Interleukin 4 (IL-4) is a pleiotropic cytokine that plays a major regulatory role in the immune system. Signal transduction of IL-4 is mediated by a sequential binding process, initiated first by binding of IL-4 to its high-affinity single membrane spanning receptor chain IL-4Rα. This intermediate ligand receptor complex then recruits one of two possible low-affinity receptor subunits, the common gamma chain (γc) or the IL-13Rα1 chain, into the functional hetero-trimeric complex to initiate signalling. The overall structure of IL-4 comprises the known four-helical bundle in up-up-down-down topology, which like the crystal packing is unaffected by these mutations.

Analysis of the variants T13D and F82D yielded dissociation constants KD of 0.02 – 0.04 nM and 0.03 – 0.04 nM respectively. The structures of the IL-4 variants T13D (max. resolution 1.65 Å), F82D (max. resolution 1.7Å) and T13D-F82D (max. resolution 1.8Å) were refined on the basis of the structure of wild-type IL-4 (max. resolution 1.8Å); all crystals were obtained under identical conditions, allowing detailed comparison. The structure of the super-agonist variant F82D shows a different picture; the side chain conformation, i.e. the χ1 and χ2 torsion angles, of Asp82 is identical to that of the wild-type Phe82. Interestingly, the high-resolution structure of variant F82D reveals two alternative side chain conformations for Arg85. In one, the side chain is not hydrogen-bonded to the Asp residue introduced at position 82 and is oriented towards the solvent. In the second, the side chain interacts with the carboxylate group of Asp82 via a weak single hydrogen bond, but it is much less fixed than in the variant T13D. The distance between the amino group of Arg85 and the carboxylate group of Asp82 is 3.2Å and therefore close to the exclusion criterion for a hydrogen bond. In addition, the temperature factors of the Arg85 side chain atoms are elevated compared to those of rigid main chain or side chain atoms in the variant F82D, indicating that the stabilization of a certain side chain conformation is not as rigid as in variant T13D. The model of the F82D:IL-4Rα complex allows us to propose a stabilizing mechanism similar to that suggested for the complex of T13D and IL-4Rα. Here, too, the carboxylate group of Asp82 (F82D) forms a bi-dentate salt bridge with the guanidinium group of Arg85, thereby immobilizing the side chain of Arg85 in the ligand-receptor interface.

> HKCDITLQEIIKTLNSLTEQKTLCTELTVTDIFAASKNTTEKETFCRAATVLRQFYSHHEKDTRCLGATAQQFHRHKQLIRDLKRLDRNLWGLAGLNSCPVKEANQSTLENFLERLKTIMREKYSKCSS One especially common junction element is the kink-turn (k-turn). k-turns are elements in double-stranded RNA that introduce a tight kink into the helical axis, with an included angle close to 50°. A standard k-turn comprises a three-nucleotide bulge followed by successive G•A and A•G trans G(sugar edge)•A(Hoogsteen edge) basepairs. k-turns are commonly-occurring motifs that introduce sharp kinks into duplex RNA, thereby facilitating tertiary contacts. Both the folding and conformation of k-turns are determined by their local sequence. k-turns fall into two conformational classes, called N3 and N1, that differ in the pattern of hydrogen bonding in the core. We show here that this is determined by the basepair adjacent to the critical G•A pairs.

We therefore decided to extend the study with a systematic structural analysis of HmKt-7 as a function of the 3b,3n sequence. This was performed in the constant environment of the SAM-I riboswitch, modified by replacing its natural k-turn by HmKt-7 with different 3b,3n sequences. In this way we could observe the effect of changing the 3b,3n sequence alone in an otherwise completely unchanged RNA molecule. Additionally, we hoped we might expand the range of 3b,3n sequences beyond the eight found in the natural k-turns to date. Six are completely new, i.e. 3b,3n = C•A, C–G, C•U, G•G, U–A and U•C, five of which adopt the N1 conformation. There is a tendency for 3b = purine to result in an N3 structure, but the generality is broken by the N1 structure adopted by the 3b,3n = G•G Kt-7 variant. Altogether seven of the new structures are in the N1 conformation, and clearly simply changing the 3b,3n sequence alone is sufficient to induce the structure of Kt-7 to change within the riboswitch environment. Evidently the 3b,3n sequence is the major determinant of the k-turn conformation.

> GGCUUAUCAAGAGAGGGGGAGCGACUGGCGCGAAGAGCCCCGGCAACCAGAAAUGGUGCCAAUUCCUGCAGCGGAAACGUUGAAAGAUGAGCCG>AAPPVQSQVDCENSQPWHVAVYRFNKYQCGGVLLDRNWVLTAAHCYNDKYQVWLGKNNFLEDEPSDQHRLVSKAIPHPDFNMSLLNEHTPQPEDDYSNDLMLLRLSKPADITDVVKPITLPTEEPKLGSTCLASGWGSTTPIKFKYPDDLQCVNLKLLPNEDCDKAHEMKVTDAMLCAGEMDGGSYTCEHDSGGPLICDGILQGITSWGPEPCGEPTEPSVYTKLIKFSSWIRETMANNP[2x];>SSTHPVFHMGEFSVCDSVSVWVGDKTTATDIKGKEVTVLAEVNINNSVFRQYFFETKCRASNPVESGCRGIDSKHWNSYCTTTHTFVKALTTDEKQAAWRFIRIDTACVCVLSRKATR[2x];>[2x]IVGGFKCEKNSQPWHVAVYRYTQYLCGGVL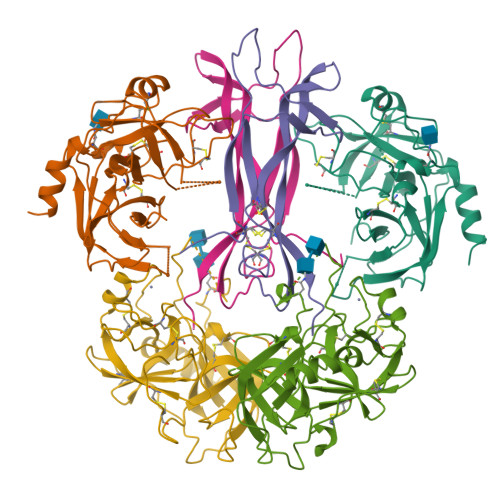LDPNWVLTAAHCYDDNYKVWLGKNNLFKDEPSAQHRFVSKAIPHPGFNMSLMRKHIRFLEYDYSNDLMLLRLSKPADITDTVKPITLPTEEPKLGSTCLASGWGSITPTKFQFTDDLYCVNLKLLPNEDCAKAHIEKVTDAMLCAGEMDGGKDTCKGDSGGPLICDGVLQGITSWGHTPCGEPDMPGVYTKLNKFTSWIKDTMAKNP> GSHMSATAATVPPAAPAGEGGPPAP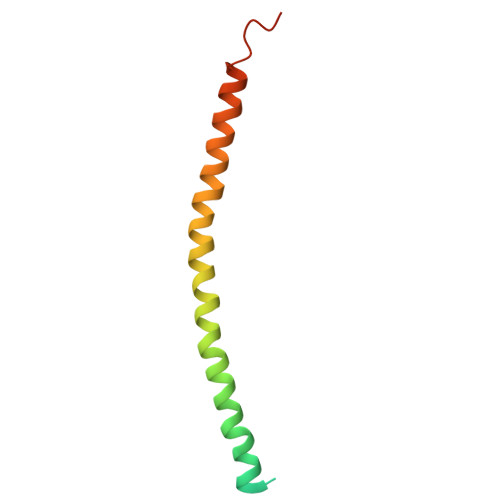PPNLTSNRRLQQTQAQVDEVVDIMRVNVDKVLERDQKLSELDDRADALQAGASQFETSAAKLKRKYWWKNLK> MSPSKLSNDETPPDLDFRFTGIKQRLIKSENVKQVTASWKRLLVEINKEFTEIAKIGPSYVPKCDFIDIKDNKLPQQVSELFKQRGCLMIENVIDVDRIDIWFNELV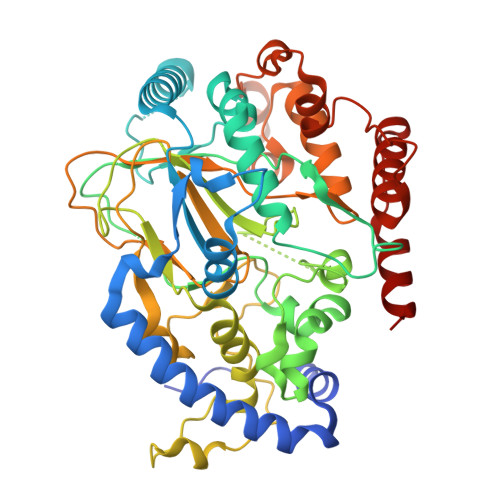EFCKTHPETAGYTFPNPTSWYNVFWSKPQTEARFHPNMKAIFKAMSKEFYVEDKENCLIDLDTQLVYGDRIRIREPGKAAALPLHLDSSSIERWEDIMYSEVYKSIFEGDWENWDAFKLDERTYSKENLYKDEDDTGGKSTICSSFRTLQGWLALSNNKSGEGTLRVLPSLKLSMAYIMLRPFFWKDPESGNIDDYEIDLITPKFPGTVPGTGQLFLDKFYPHLHQGIISIPDVKKGSFVFWHCDLPHEVDREHNGNGHSSVLYYGQTPLSITNIQTLLDTRDAFLKNISPADYRSQLNEEEKQKEFQGANIDDLKNDIDSKRSMGLEEFEKPENMSGGQAKIRSIANQALKSSGFNVDKYIHHAAKLE>SKKHTGYVGLKNQGATCYMNSLLQTLFF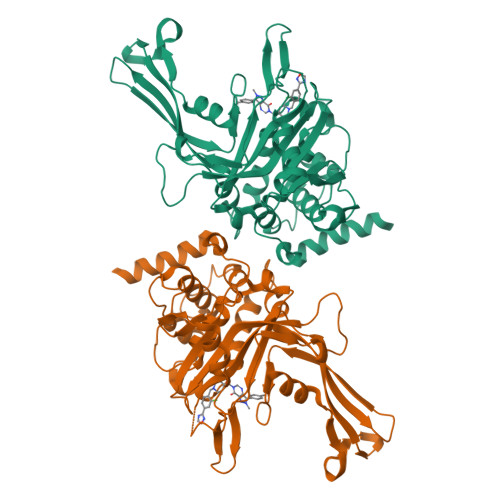TNQLRKAVYMMPTEGDDSSKSVPLALQRVFYELQHSDKPVGTKKLTKSFGWETLDSFMQHDVQELCRVLLDNVENKMKGTCVEGTIPKLFRGKMVSYIQCKEVDYRSDRREDYYDIQLSIKGKKNIFESFVDYVAVEQLDGDNKYDAGEHGLQEAEKGVKFLTLPPVLHLQLMRFMYDPQTDQNIKINDRFEFPEQLPLDEFLQKTDPKDPANYILHAVLVHSGDNHGGHYVVYLNPKGDGKWCKFDDDVVSRCTKEEAIEHNYGGHDDDLSVRHCTNAYMLVYIRESKLSEVLQAVTDHDIPQQLVERLQEEKRIEAQK[2x]>[2x]MSEKTT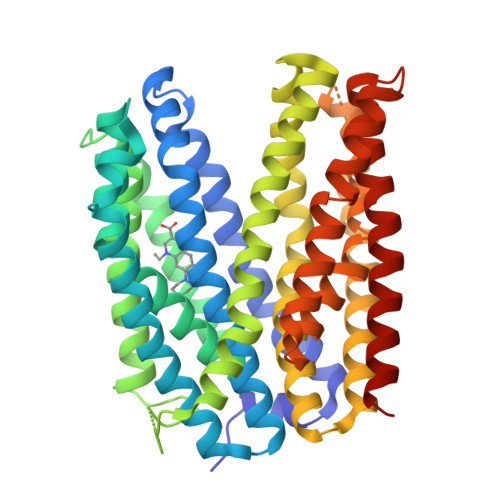KGVQLLRGDPKKAIVRLSIPMMIGMSVQTLYNLADGIWVSGLGPESLAAVGLFFPVFMGIIALAAGLGVGTSSAIARRIGARDKEGADNVAVHSLILSLILGVTITITMLPAIDSLFRSMGAKGEAVELAIEYARVLLAGAFIIVFNNVGNGILRGEGDANRAMLAMVLGSGLNIVLDPIFIYTLGFGVVGAAYATLLSMVVTSLFIAYWLFVKRDTYVDITLRDFSPSREILKDILRVGLPSSLSQLSMSIAMFFLNSVAITAGGENGVAVFTSAWRITMLGIVPILGMAAATTSVTGAAYGERNVEKLETAYLYAIKIAFMIELAVVAFIMLFAPQVAYLFTYSESAQVIKGDLISALRTLPVFLVLTPFGMMTSAMFQGIGEGEKSLILTIFRTLVMQVGFAYIFVHYTTLGLRGVWIGIVIGNMVAAIVGFLWGRMRISALKKTSATGGKR>[2x]ASAWPEEKNYHQPAILNSSALRQIAEGTSISEMWQNDLQPLLIERYPGSPGSYAARQHIMQRIQRLQADWVLEIDTFLSQTP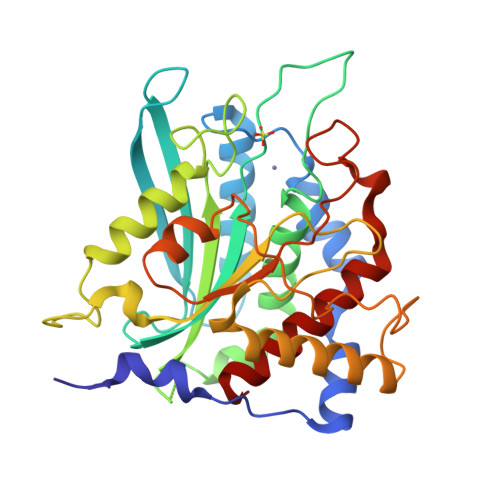YGYRSFSNIISTLNPTAKRHLVLACHYDSKYFSHWNNRVFVGATDSAVPCAMMLELARALDKKLLSLKTVSDSKPDLSLQLIFFDGEEAFLHWSPQDSLYGSRHLAAKMASTPHPPGARGTSQLHGMDLLVLLDLIGAPNPTFPNFFPNSARWFERLQAIEHELHELGLLKDHSLEGRYFQNYSYGGVIQDDHIPFLRRGVPVLLLIPSPFPEVWHTMDDNEENLDESTIDNLNKILQVFVLEYLHL>MEVNKKQLADIFGASIRTIQNWQEQGMPVLRGGGKGNEVLYDSAAVIKW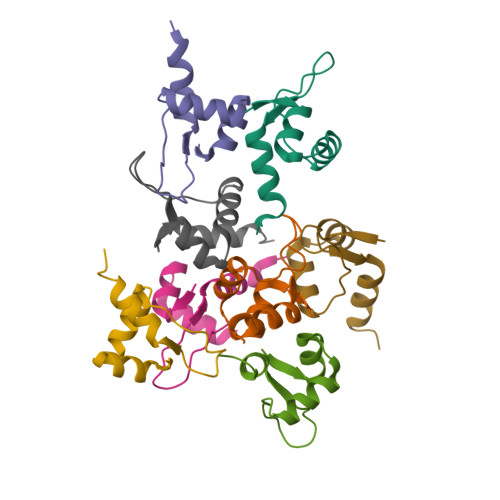YAERDAC[8x]> GSKGNIRVIARVRPVTKEDGEGPEATNAVTFDADDDSIIHLLHKGKPVSFELDKVFSPQASQQDVFQEVQALVTSCIDGFNVCIFAYGQTGAGKTYTMEGTAENPGINQRALQLLFSEVQEKASDWEYTIT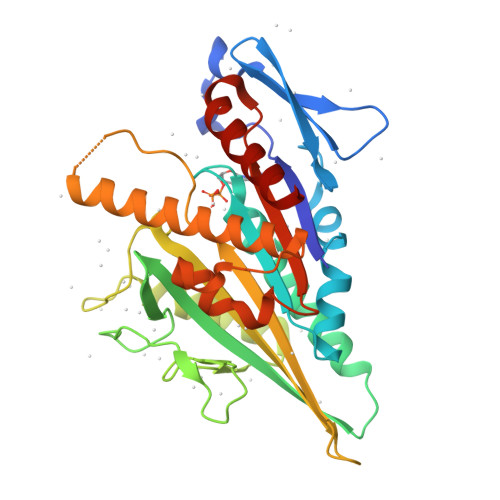VSAAEIYNEVLRDLLGKEPQEKLEIRLCPDGSGQLYVPGLTEFQVQSVDDINKVFEFGHTNRTTEFTNLNEHSSRSHALLIVTVRGVDCSTGLRTTGKLNLVDLAGSERVGKSGAEGSRLREAQHINKSLSALGDVIAALRSRQGHVPFRNSKLTYLLQDSLSGDSKTLMVVQVSPVEKNTSETLYSLKFAERVRSVEL> MSSHTATKYDVFLSFR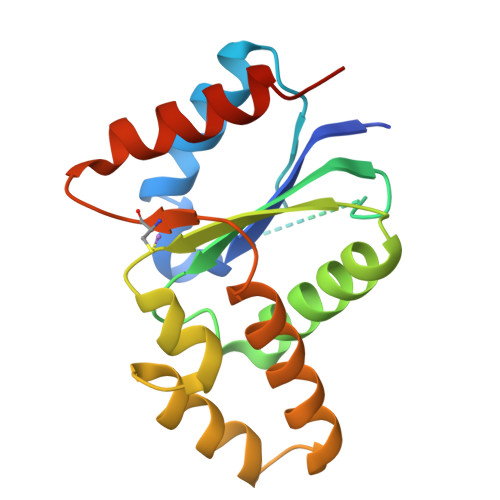GHDTRHNFISFLYKELVRRSIRTFKDDKELENGQRFSPELKSPIEVSRFAVVVVSENYAASSWCLDELVTIMDFEKKGSITVMPIFYGVEPNHVRWQTGVLAEQFKKHASREDPEKVLKWRQALTNFAQLSGDCSGDDDSKLVDKIANEISNKKTIYATI>[2x]GSHMQNIPIKRINVPEIGIATELSHGVVQVQFYDGSVVS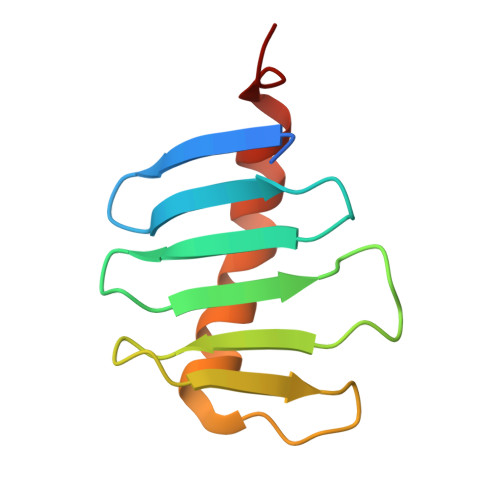VIPSMQGGGITYTQPNGTSTHFGKGDDLPFPVRDRVGQIPNIQLKLKTAPLLGS> LTLGNTTSSVILTNYMDTQYYGEIGIGTPPQTFKVVFDTGSSNVWVPSSKCSRLYTACVYHKLFDASDSSSYKHNGTELTLRYSTGTVSGFLSQDIITVGGITVTQMFGEVTEMPALPFMLAEFDGVVGMGFIEQAIGRVTPIFDNIISQGVLKEDVFSFYYNRDSLGGQIVLGGSDPQHYEGNFHYINLIKTGVWQIQMKGVSVGSSTLLCEDGCLALVDTGASYISGSTSSIEKLMEALGAKKRLFDYVVKCNEGPTLPDISFHLGGKEYTLTSADYVFQESYSSKKLCTLAIHAMDIPPPTGPTWALGAT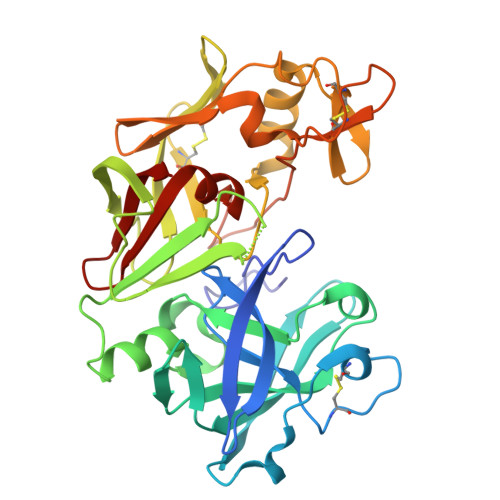FIRKFYTEFDRRNNRIGFALAR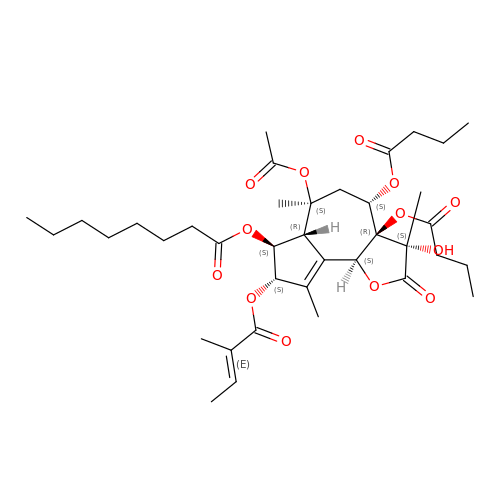(3S,3aR,4S,6S,6aR,7S,8S,9bS)-6-(acetyloxy)-3a,4-bis(butanoyloxy)-3-hydroxy-3,6,9-trimethyl-8-{[(2E)-2-methylbut-2-enoyl]oxy}-2-oxo-2,3,3a,4,5,6,6a,7,8,9b-decahydroazuleno[4,5-b]furan-7-yl octanoate | C38 H56 O13 | ARWTVHVQANENHV-XDRCOMTCSA-N6,8-diamino-7-chloro-1-methyl-2-oxo-1,2-dihydropyrrolo[4,3,2-de]quinoline-4-carboxamide | C12 H10 Cl N5 O2 | 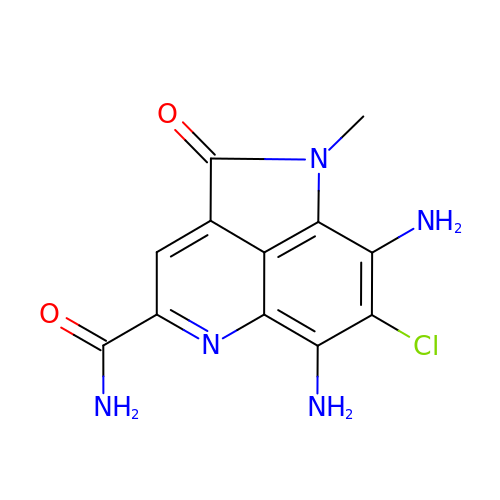HWRGTOQGZGTNID-UHFFFAOYSA-N> GNNVVVLGTQWGDEGKGKIVDLLTERAKYVVRYQGGHNAGHTLVINGEKTVLHLIPSGILRENVTSIIGNGVVLSPAALMKEMKELEDRGIPVRERLLLSEACPLILDYHVALDNAREKARGAKAIGTTGRGIGPAYEDKVARRGLRVGDLFDKETFAEKLKEVMEYHNFQLVNYYKAEAVDYQKVLDDTMAVADILTSMVVDVSDLLDQARQRGDFVMFEGAQGTLLDIDHGTYPYVTSSNTTAGGV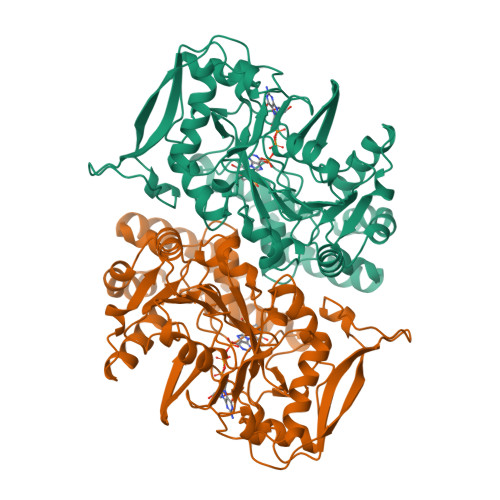ATGSGLGPRYVDYVLGILKAYSTRVGAGPFPTELFDETGEFLCKQGNEFGATTGLRRRTGWLDTVAVRRAVQLNSLSGFCLTKLDVLDGLKEVKLCVAYRMPDGREVTTTPLAADDWKGVEPIYETMPGWSESTFGVKDRSGLPQAALNYIKRIEELTGVPIDIISTGPDRTETMILRDPFDA>[2x]MKMLEQLEKKLGYTFKDKS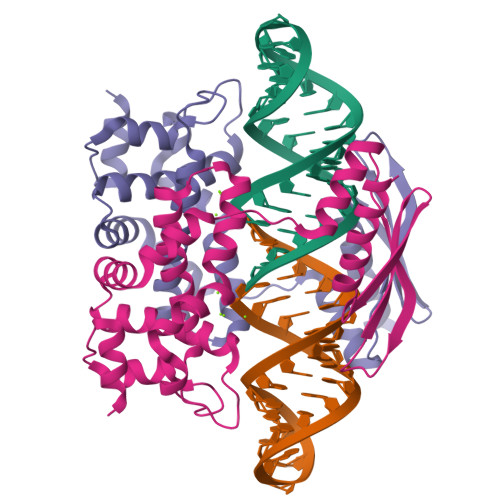LLEKALTHVSYSKKEHYETLEFLGDALVNFFIVDLLVQYSPNKREGFLSPLKAYLISEEFFNLLAQKLELHKFIRIKRGKINETIIGDVFEALWAAVYIDSGRDANFTRELFYKLFKEDILSAIKEGRVKKDYKTILQEITQKRWKERPEYRLISVEGPHHKKKFIVEAKIKEYRTLGEGKSKKEAEQRAAEELIKLLEESE> GPAPADPGKAGVPGVAAPGAPAAAPPA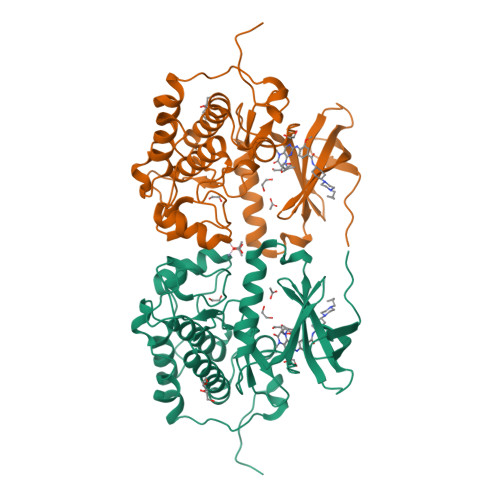KEIPEVLVDPRSRRRYVRGRFLGKGGFAKCFEISDADTKEVFAGKIVPKSLLLKPHQREKMSMEISIHRSLAHQHVVGFHGFFEDNDFVFVVLELCRRRSLLELHKRRKALTEPEARYYLRQIVLGCQYLHRNRVIHRDLKLGNLFLNEDLEVKIGDFGLATKVEYDGERKKVLCGTPNYIAPEVLSKKGHSFEVDVWSIGCIMYTLLVGKPPFETSCLKETYLRIKKNEYSIPKHINPVAASLIQKMLQTDPTARPTINELLNDEFFTSGYIPARLPITCLTIPPRFSIAPSSLDPSNRKPLTVLNK3,6-anhydro-beta-L-galactopyranose | C6 H10 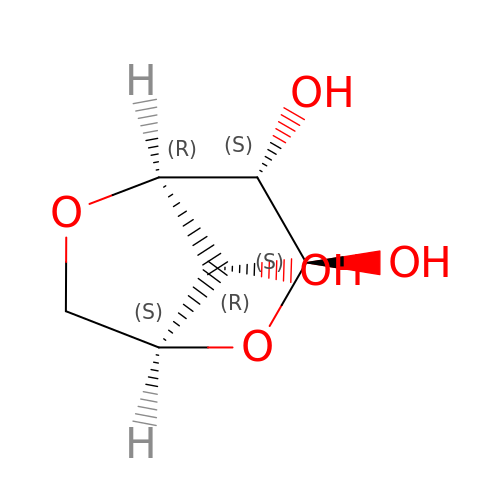O5 | DCQFFOLNJVGHLW-ZSNZIGRDSA-N>HPKLVSSTPAEGSEGAAPAKIELHFSENLVTQFSGAKLVMTAMPGMEHSPMAVKAAVSGGGDPKTMVITPASPLTAGTYK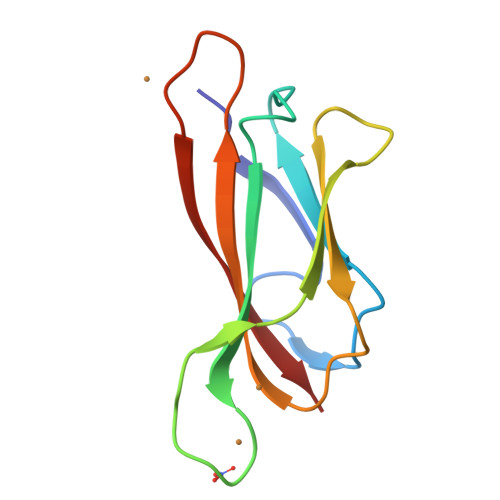VDWRAVSSDTHPITGSVTFKVK[3x]>[2x]MADSELQLVEQRIRSFPDFPTPGVVFRDISPVLKDPASFRAAIGLLARHLKATHGGRIDYIAGLDSRGFLFGPSLAQELGLGCVLIRKRGKLPGPTLWASYSLEYGKAELEIQKDALEPG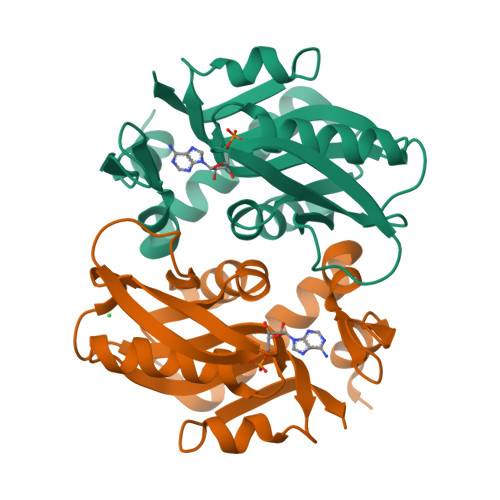QRVVVVDDLLATGGTMNAACELLGRLQAEVLECVSLVELTSLKGREKLAPVPFFSLLQYE> MTTPTMQSTSLLTEHLGYPPISLVDDIINAVNEIMYKCTNAMEKYLMQRNIIGKKDFSDEIKIGTAKLESLLE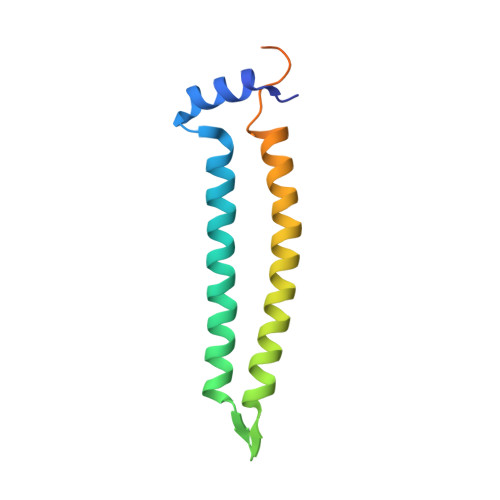NSVDKNFDKLELYVLRNILSIPSDLLEENRFRLLHHEKLVLTDSATR> GMPLKPEEHEDILNKLLDPELAQSERTEALQQLRVNYGSCVSEYNDLTKSLARERDTSRRLLAEKEREMAEMRARMQQQLDEYQELLDIKLALDMEIHAYRKLLEGEEERL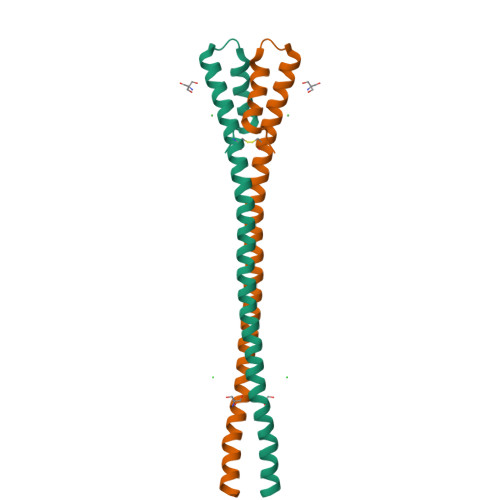RLSPSPTSQRSRGRAS Muscle-specific RING fingers proteins (MuRFs) are E3 ubiquitin ligases that associate with the sarcomeric cytoskeleton reportedly through their CC domains. MuRFs form the C-II TRIM class, whose C-terminal specific fraction contains a COS (C-terminal subgroup One Signature)-box motif and an intrinsically disordered acidic tail. MuRF1 targets components of the contractile sarcoskeleton; namely, myosin, troponin-T and titin. Despite their functional diversity, TRIM proteins invariably share a tripartite fold consisting of a RING finger (R), one or two RING finger-like B-box domains (B) and a helical segment predicted to form a coiled-coil (CC) motif.

To gain an insight into the assembly of the CC-prone segment identified, we elucidated the crystal structure of the corresponding fragment from human MuRF1 (MuRF1CC) to 2.1 Å resolution. The crystals contained four copies of the MuRF1CC chain in their asymmetric unit. These assembled into two parallel dimers, each having an ‘open scissor’ conformation that intercalated through their C-terminal ends to form a palindromic, inverted tetramer. In MuRF1, however, the chains within each dimer are out of registry by one full heptad-repeat and their crossing angle is broad, leading to the unpairing of both N- and C-termini. The resulting exposure of hydrophobic residues at the C-terminus permits the formation of an interchain hydrophobic core that supports the assembly of the inverted tetramer. Other than that core, the contacts within each dimer are few, with only two salt bridges (K224-E236’ and E236-K238’) providing chain recognition (analysis of chain interfaces used PISA). One additional salt bridge (K238-D268’’; chains DA in figure 3a) is present in the structure, but it contributes to tetramer stabilization. The analysis revealed that MuRF1CC can establish manifold interactions, being able to support concurrently the formation of parallel and antiparallel dimers and tetrameric helical bundles. In the MuRF1CC tetramer, helices arrange themselves along the same interfaces as those occupied by the COS-box α-hairpin in the ab initio models.

>[4x]GAMDTLYAILDEKKSELLQRITQEQEEKLSFIEALIQQYQEQLDKSTKLVETAIQSLDEPG>MKAHPKEMVPLMGKRVAAPSGNPAVLPEKRPAEITPTKKSAHFFLEIEGFEPNPTVAKTSPPVFSKPMDSNIRQCISGNCDDMDSPQSPQDDVTETPSNPNSPSAQLAKEEQRRKKRRLKKRIFAAVSEGCVEELVELLVELQELCRRRHDEDVPDFLMHKLTASDTGATCLMKALLNINPNTKEIVRILLAFAEENDILGRFINAEYTEEAYEGQTALNIAIERRQGDIAALLIAAGADVNAHAKGAFFNPKYQHEGFYFGETPLALAACTNQPEIVQLLMEHEQTDITSRDSRGNNILHALVTVAEDFKTQNDFVKRMYDMILLRSGNWELETTRNNDGLTPLQLAAKMGKAEILKYILSREIKEKRLRSLSRKFTDWAYGPVSSSLYDLTNVDTTTDNSVLEITVYNTNIDNRHEMLTLEPLHTLLHMKWKKFAKHMFFLSFCFYFFYNITLTLVSYYRPREEEAIPHPLALTHKMGWLQLLGRMFVLIWAMCISVKEGIAIFLLRPSDLQSILSDAWFHFVFFIQAVLVILSVFLYLFAYKEYLACLVLAMALGWANMLYYTRGFQSMGMYSVMIQKVILHDVLKFLFVYIVFLLGFGVALASLIEKCPKDNKDCSSYGSFSDAVLELFKLT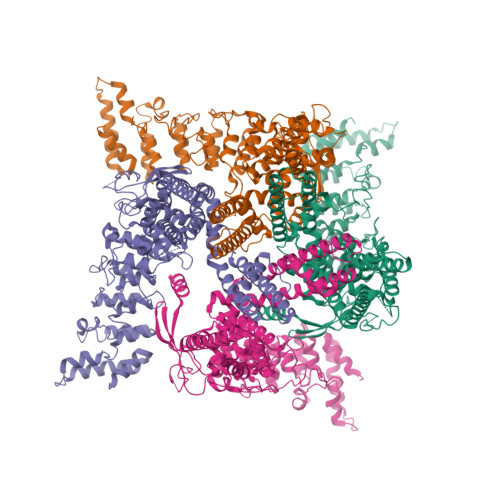IGLGDLNIQQNSKYPILFLFLLITYVILTFVLLLNMLIALMGETVENVSKESERIWRLQRARTILEFEKMLPEWLRSRFRMGELCKVAEDDFRLCLRINEVKWTEWKTHVSFLNEDPGPVRRTDFNKIQDSSRNNSKTTLNAFEEVEEFPETSV[4x]>MDYRQLHRWDLPPEEAIKVQNELRKKIKLTPYEGEPEYVAGVALSFPGKEEGLAVIVVLEYPSFKILEVVSERGEITFPYIPGLLAFREGPLFLKAWEKLRTKPDVVVFDGQGLAHPRKLGIASHMGLFIEIPTIGVAKSRLYGTFKMPEDKRCSWSYLYDGEEIIGCVIRTKEGSAPIFVSPGHLMDVESSKRLIKAFTLPGRRIPEPTRLAHIYTQRLKKGLF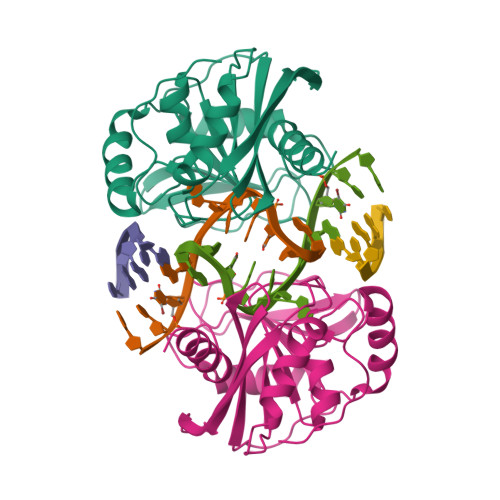[2x]>MIMEELAKKIEEEILNHVREPQIPDREVNLLDFGARGDGRTDCSESFKRAIEELSKQGGGRLIVPEGVFLTGPIHLKSNIELHVKGTIKFIPDPERYLPVVLTRFEGIELYNYSPLVYALDCENVAITGSGVLDGSADNEHWWPWKGKKDFGWKEGLPNQQEDVKKLKEMAERGTPVEERVFGKGHYLRPSFVQFYRCRNVLVEGVKIINSPMWCIHPVLSENVIIRNIEISSTGPNNDGIDPESCKYMLIEKCRFDTGDDSVVIKSGRDADGRRIGVPSEYILVRDNLVISQASHGGLVIGSEMSGGVRNVVARNNVYMNVERALRLKTNSRRGGYMENIFFIDNVAVNVSEEVIRINLRYDNEEGEYLP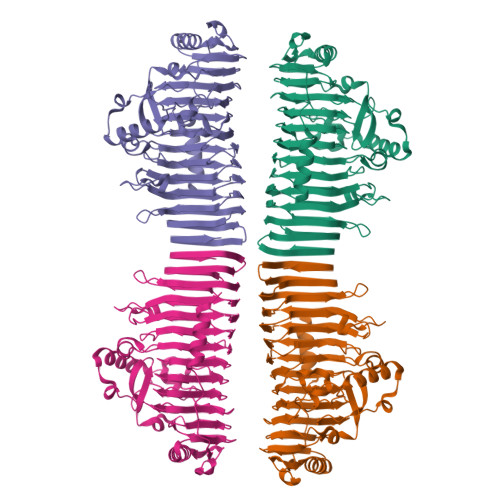VVRSVFVKNLKATGGKYAVRIEGLENDYVKDILISDTIIEGAKISVLLEFGQLGMENVIMNGSRFEKLYIEGKALLK[4x]>[7x]MGSSHHHHHHHHHHSSGLVPAGSMTQSQTVTVDQQEILNRANEVEAPMADPPTDVPITPCELTAAKNAAQQLVLSADNMREYLA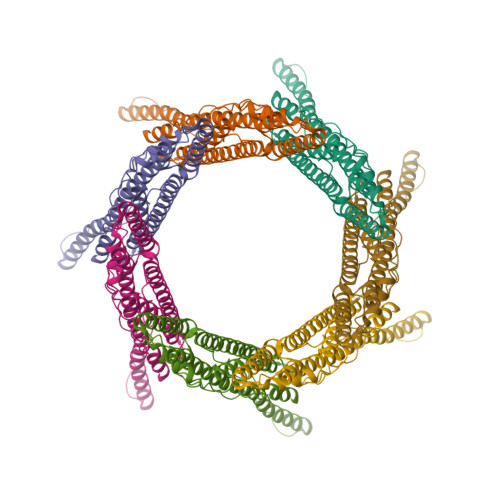AGAKERQRLATSLRNAAKAYGEVDEEAATALDNDGEGTVQAESAGAVGGDSSAELTDTPRVATAGEPNFMDLKEAARKLETGDQGASLAHFADGWNTFNLTLQGDVKRFRGFDNWEGDAATACEASLDQQRQWILHMAKLSAAMAKQAQYVAQLHVWARREHPTYEDIVGLERLYAENPSARDQILPVYAEYQQRSEKVLTEYNNKAALEPVNPPKPPPAIKIDPPPPPQEQGLIPGFLMPPSDGSGVTPGTGMPAAPMVPPTGSPGGGLPADTAAQLTSAGREAAA>MNNDVFPNKFKAALAAKQVQIGCWSALSNPISTEVLGLAGFDWLVLDGEHAPNDISTFIPQLMALKGSASAPVVRVPTNEPVIIKRLLDIGFYNFLIPFVETKEEAELAVASTRYPPEGIRGVSVSHRANMFGTVADYFAQSNKNITILVQIESQQGVDNVDAIAATEGVDGIFVGPSDLAAA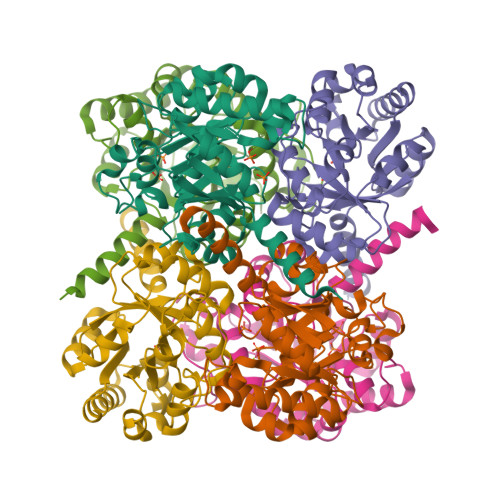LGHLGNASHPDVQKAIQHIFNRASAHGKPSGILAPVEADARRYLEWGATFVAVGSDLGVFRSATQKLADTFKK[2x]(2E)-3-(1H-IMIDAZOL-4-YL)ACRYLIC 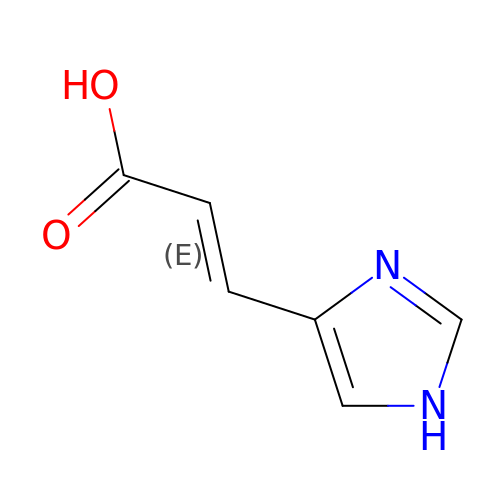ACID | C6 H6 N2 O2 | LOIYMIARKYCTBW-OWOJBTEDSA-N>[3x]MKFKHQGLVADLLPNIRVMQGVGHFMFNYYSEGKKFPHRIYCIVTLLLLLLQYGMMAVNLMMESDDVDDLTANTITMLFFLHPIVKMIYFPVRSKIFYKTLAIWNNPNSHPLFAESNARFHALAITKMRRLLFCVAGATIFSVISWTGITFIEDSVKRITDPETNETTIIPIPRLMIRTFYPFNAMSGAGHVFALIYQFYYLVISMAVSNSLDVLFCSWLLFACEQLQHLKAIMKPLMELSATLDTVVPNSGELFKAGSADHLRESQGVQPSGNGDNVLDVDLRGIYSNRQDFTATFRPTAGTTFNGGVGPNGLTKKQEMLVRSAIKYWVERHKHVVRLVTAVGDAYGVALLLHMLTTTITLTLLAYQATKVNGVNVYAATVIGYLLYTLGQVFLFCIFGNRLIEESSSVMEAAYSCHWYDGSEEAKTFVQIVCQQCQKAMSISGAKFFTVSLDLFASVLGAVVTYFMVLVQLK;> MASILDCPIVSVNARVWRFWSFVLKHDAMRYISIIPVTVMTFFMFTDLCRSWGNIQELIIKAYFAVLYFNAVLRTLILVKDRKLYENFMQGISNVYFEISHIDDHKIQSLLKSYTVRARMLSISNLALGAIISTCFVVYPIFTGERGLPYGMFIPGLDSFRSPHYEIIYIVQVVLTFPGCCMYIPFTSFFASTTLFGLVQIKTLQRQLQTFKDNINSQDKEKVKAKVVKLIEDHKRIITYVSELNSLVTYICFVEFLSFGMMLCALLFLLNVIENHAQIVIVAAYIFMIISQIFAFYWHANEVREESMNLAEAAYSGPWVELDNSIKKKLLLIILRAQQPLEITVGNVYPMTLEMFQSLLNASYSYFTLLRRVYN

Most insects, including human-targeting mosquitoes, detect odors through odorant-activated ion channel complexes consisting of a divergent odorant-binding subunit (OR) and a conserved co-receptor subunit (Orco). As a basis for understanding how odorants activate these heteromeric receptors, we report here cryo-EM structures of two different heteromeric odorant receptor complexes containing ORs from disease-vector mosquitos Aedes aegypti or Anopheles gambiae. We determined the structure of a heteromeric complex formed by ORs from these species in complex with a Apocrypta bakeri fig wasp Orco that is amenable to structural determination. We find that these complexes form asymmetric tetramers containing 1 OR and 3 Orco subunits, where activation of the sole OR subunit upon ligand binding suffices to open the ion conduction pathway.

We first focused on the conserved OR10 receptor family, which detects indole and derivatives in various mosquito species. We corroborated the functionality of the AaOR10/Orco complexes by heterologously expressing these complexes in cultured HEK293 cells and performing voltage-clamp electrophysiology to measure their response to indole and o-cresol, canonical odorants known to activate AaOR10 heteromers. We therefore determined the cryo-EM structure of the AaOR10/Orco complex bound to o-cresol to an overall resolution of 2.9 Å. The OR10 S7b helix shifts diagonally outwards from the main channel axis, increasing the distance to the opposing Orco subunit from 6.2 Å to 9.7 Å. A conformational change in the OR subunit alone is sufficient to open the pore of the AaOR10/Orco complex. Therefore, the presence of the OR subunit is sufficient to impart odorant specificity to the complex and lead to channel opening without any concerted movement of the other subunits. Mutation of these residues to alanine decreases the apparent affinity of o-cresol activation, seen as a right-shift in the dose-response curve assessed using an established calcium flux functional assay. In the o-cresol bound structure, density corresponding to the hypothetical lipid is absent. In summary, by destabilizing the inactive conformation and stabilizing the active conformation, o-cresol shifts the receptor conformational equilibrium towards the active state, resulting in pore opening.> ASLPPLEWPLSSQSGSYELRIEVQPKPHHRAHYETEGSRGAVKAPTGGHPVVQLHGYMENKPLGLQIFIGTADERILKPHAFYQVHRITGKTVTTTSYEKIVGNTKVLEIPLEPKNNMRATIDCAGILKLRNADIELRKGETDIGRKNTRVRLVFRVHIPESSGRIVSLQTASNPIECSQRSAHELPMVE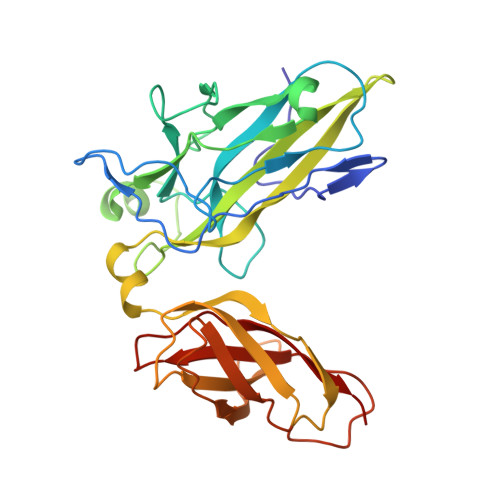RQDTDSCLVYGGQQMILTGQNFTSESKVVFTEKTTDGQQIWEMEATVDKDKSQPNMLFVEIPEYRNKHIRTPVKVNFYVINGKRKRSQPQHFTYHPV>[4x]MAEKMQAIMKTKPAYGAELVEVDVPKPGPGEVLIKVLATSICGTDLHIYEWNEWAQSRIKPPQIMGHEVAGEVVEVGPGVEDLQVGDYISVETHIVCGKCYACKHNRYHVCQNTKIFGVDMDGVFAHYAIVPAKNAWKNPKDMPPEYAALQEPLGNAVDTVLAGPIAGRSTLITGAGPLGLLGIAVAKASGAYPVIVSEPSEFRRKLAKKVGADYVVNP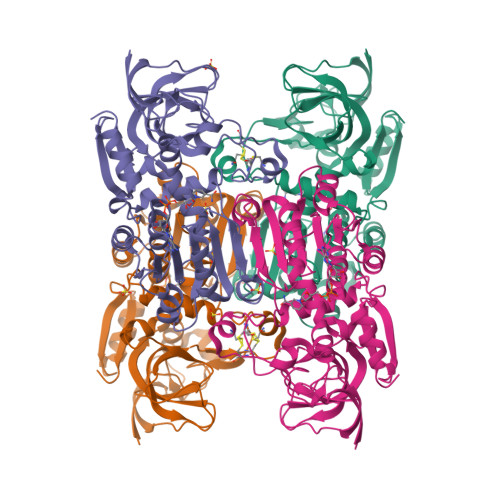FEEDPVKFVMDITDGAGVEVFLEFSGAPKALEQGLKAVTPGGRVSLLGLFPREVTIDFNNLIIFKALEVHGITGRHLWETWYTVSSLIQSGKLNLDPIITHKYKGFDKFEEAFELMRAGKTGKVVFFPHKG>[4x]IHIGAIFDESAKKDDEVFRTAVGDLNQNEEILQTEKITFSVTFVDGNNPFQAVQEACELMNQGILALVSSIGCTSAGSLQSLADAMHIPHLFIQRSTAGTPRSGCGLTRSNRNDDYTLSVRPPVYLHDVILRVVTEYAWQKFIIFYDSEYDIRGIQEFLDKVSQQGMDVALQKVENNINKMITTLFDTMRIEELNRYRDTLRRAILVMNPATAKSFITEVVETNLVAFDCHWIIINEEINDVDVQELVRRSIGRLTIIRQTFPVPQNISQRCFRGNHRISSTLCDPKDPFAQNMEISNLYIYDTVLLLANAFHKKLEDRKWHSMASLSCIRKNSKPWQGGRSMLETIKKGGVSGLTGELEFGENGGNPNVHFEILGTNYGEELGRGVRKLGCWNPVTGLNGS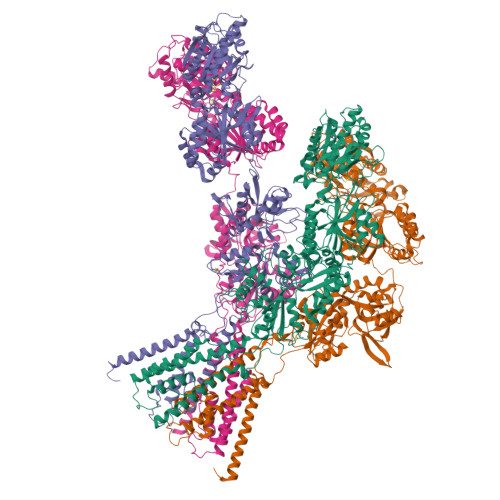LTDKKLENNMRGVVLRVVTVLEEPFVMVSENVLGKPKKYQGFSIDVLDALSNYLGFNYEIYVAPDHKYGSPQEDGTWNGLVGELVFKRADIGISALTITPDRENVVDFTTRYMDYSVGVLLRRAEKTVDMFACLAPFDLSLWACIAGTVLLVGLLVYLLNWLNPPRLQMGSMTSTTLYNSMWFVYGSFVQQGGEVPYTTLATRMMMGAWWLFALIVISSYTANLAAFLTITRIESSIQSLQDLSKQTEIPYGTVLDSAVYEHVRMKGLNPFERDSMYSQMWWMINRSNGSENNVLESQAGIQKVKYGNYAFVWDAAVLEYVAINDPDCSFYTIGNTVADRGYGIALQHGSPYRDVFSQRILELQQNGDMDILKHKWWPKNGQCDLYSSVDTKQKGGALDIKSFAGVFCILAAGIVLSCFIAMLETWWNKRKGSR>LTEQPNWLMQRAQLTPERIALIYEDQTVTFAELFAASKRMAEQLAAHSVRKGDTAAILLQNRAEMVYAVHACFLLGVKAVLLNTKLSTHERLFQLEDSGSGFLLTDSSFEKKEYEHIVQTIDVDELMKEAAEEIEIEAYMQMDATATLMYTSGTTGKPKGVQQTFGNHYFSAVSSALNLGITEQDRWLIALPLFHISGLSALFKSVIYGMTVVLHQRFSVSDVLHSINRHEVTMISAVQTMLASLLEETNRCPESIRCILLGGGPAPLPLLEECREKGFPVFQSYGMTETCSQIVTLSPEFSMEKLGSAGKPLFSCEIKIERDGQVCEPYEHGEIMVKGPNVMKSYFNRESANEASFQNGWLKTGDLGYLDNEGFLYVLDRRSDLIISGGENIYPAEVESVLLSHPAVAEAGVSGAEDKKWGKVPHAYLVLHK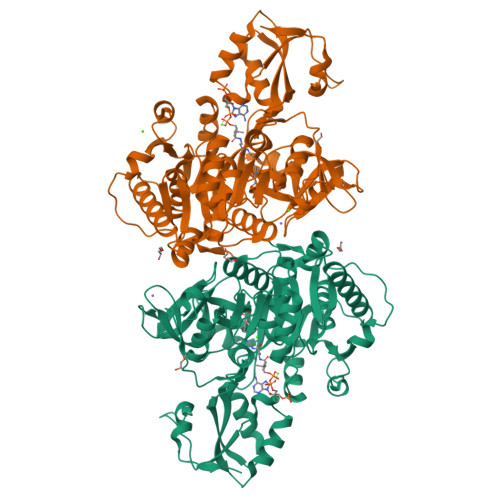PVSAGELTDYCKERLAKYKRPKKFFVLDRLPRNASNKLLRNQLKDARKGELL[4x]>[6x]MAKLITLGEILIEFNALSPGPLRHVSYFEKHVAGSEANYCVAFIKQGNECGIIAKVGDDEFGYNAIEWLRGQGVDVSHMKIDPSAPTGIFFIQRHYPVPLKSESIYYRKGSAGSKLSPED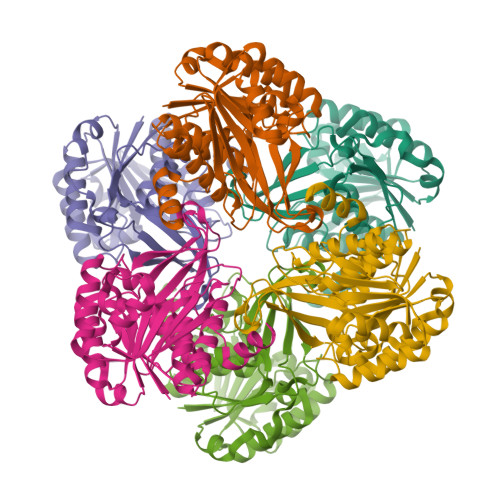VDEEYVKSADLVHSSGITLAISSTAKEAVYKAFEIASNRSFDTNIRLKLWSAEEAKREILKLLSKFHLKFLITDTDDSKIILGESDPDKAAKAFSDYAEIIVMKLGPKGAIVYYDGKKYYSSGYQVPVEDVTGAGDALGGTFLSLYYKGFEMEKALDYAIVASTLNVMIRGDQENLPTTKDIETFLREMKK>[5x]TPQNITDLCAEYHNTQIHTLNDKIFSYTESLARK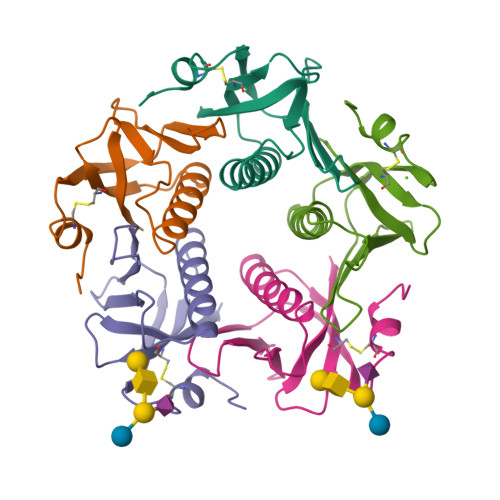REMAIITFKNGATFQVEVPGSQHIDSQKKAIERMKDTLRIAYLTEAKVEKLCVWNNKTPHAIAAISMAN>[2x]MKTLIEIKQTPDGIIKADKVFNKVKDKISLPNRILYLGCGSSHFLSKLLAMVTNMHGGLGIALPCSEFLYSKETYPIGEVELAVGISRSGETTEILLALEKINVKKLGITTRESSLTRMCDYSLVVPAIEESVVMTHSFTSFYFAYLQLLRYSYGLPPLNAGEISKATEKSLEYERYIREIVESFDFQNIIFLGSGLLYPVALEASLKMKEMSIFWSEAYPTFEVRHGFKAIADEKT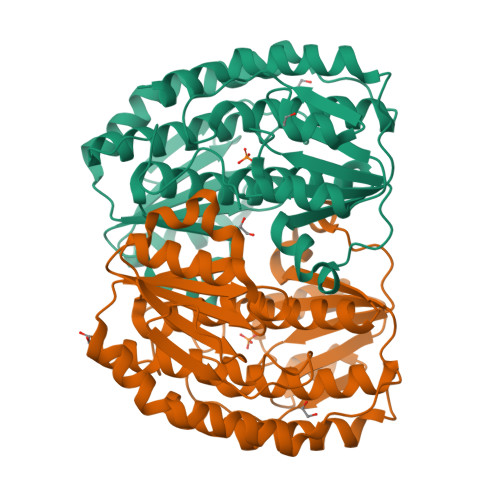LVVLMVEEPFEWHEKLVKEFKNQGAKVLVISNSPQDLGQDYSIELPRLSKDANPIPYLPIVQLLSYYKAVSRGLNPDNPRFLDKVVRW> KETAAAKFERQHMDSSTSAASSSNYCNQMMKSRNLTKDRCKPVNTFVHESLADVQAVCSQKNVACKNGQTN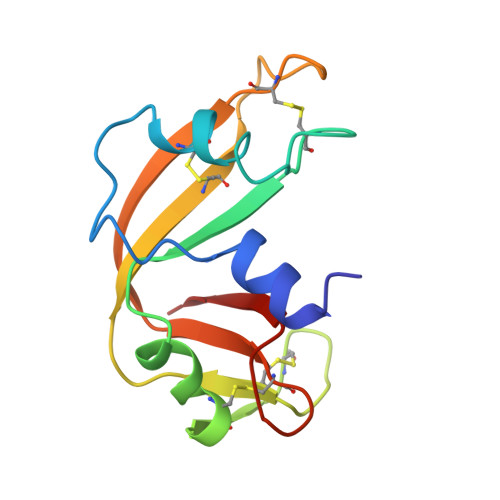CYQSYSTMSITDCRETGSSKYPNCAYKTTQANKHIIVACEGNPYVPVHFDASV> ADVVTYENKKGNVTFDHKAHAEKLGCDAC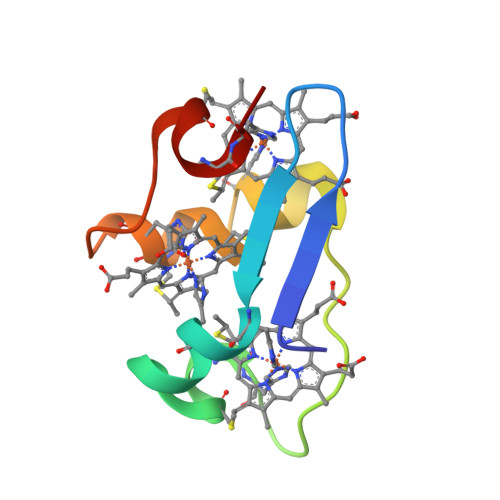HEGTPAKIAIDKKSAHKDACKTCHKSNNGPTKCGGCHIK> GSHMASMKKKGSVVIVGRINLSGDTAYAQQTRGEEGCQETSQTGRDKNQVEGEVQIVSTATQTFLATSINGVLWTVYHGAGTRTIASPKGPVTQMYTNVDKDLVGWQAPQGS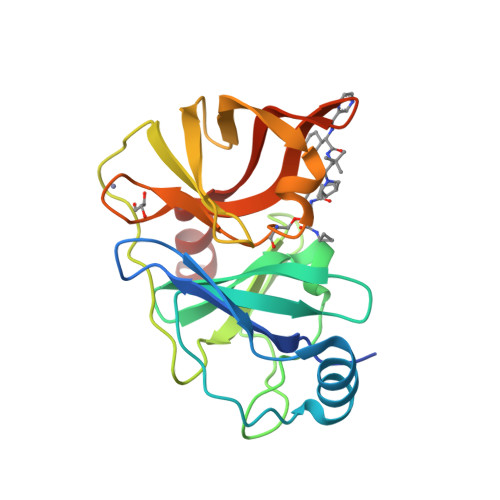RSLTPCTCGSSDLYLVTRHADVIPVRRRGDSRGSLLSPRPISYLKGSSGGPLLCPAGHAVGIFRAAVSTRGVAKAVAFIPVESLETTMRSP> GSATASDSTRRVSVRDKLLVKEVAELEANLPCTCKVHFPDPNKL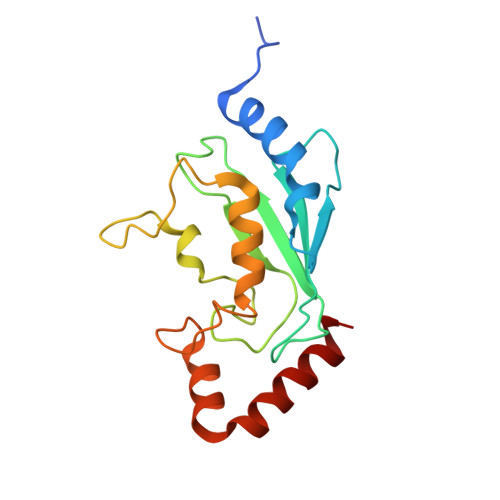HCFQLTVTPDEGYYQGGKFQFETEVPDAYNMVPPKVKCLTKIWHPNITETGEICLSLLREHSIDGTGWAPTRTLKDVVWGLNSLFTDLLNFDDPLNIEAAEHHLRDKEDFRNKVDDYIKRYAR(1~{R},3~{R},4~{S},5~{R})-3-methyl-1,3,4,5-tetrakis(oxidanyl)cyclohexane-1-carboxylic 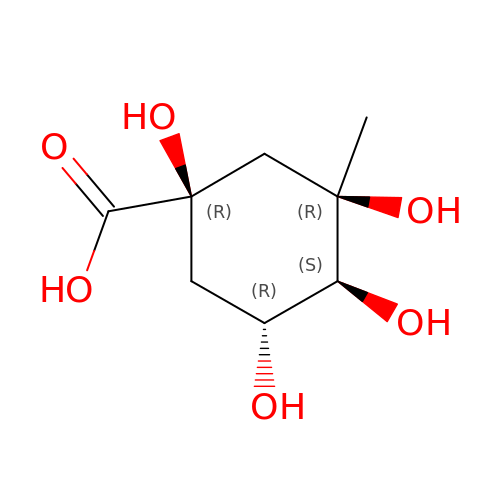acid | C8 H14 O6 | AQOKFKYCBLFIKH-IXROVEORSA-N A HEPN (higher eukaryote and prokaryote nucleotide binding) nuclease Las1 and a polynucleotide kinase Grc3 assemble into a tetramerase responsible for rRNA maturation. Las1 and Grc3 are highly conserved proteins and have recently been identified as core enzymes involved in processing and removing ITS2 spacer, which is a key step in the synthesis of 60S ribosomal subunit. Recent studies have demonstrated that Las1 is an endoribonuclease that contains a HEPN (higher eukaryote and prokaryote nucleotide binding) domain responsible for rRNA processing. Grc3 is a polynucleotide kinase responsible not only for Las1 nuclease activation, but also for nonspecific phosphorylation of the 5′-OH of the 26S pre-rRNA produced by Las1 cleavage, providing a signal for further processing by Rat1-Rai1 exonuclease.

After screening a large number of crystallization conditions, we successfully obtained well-ordered crystals of the CjLas1 HEPN domain and determined its structure at 1.80 Å resolution using molecular replacement method. The crystallographic asymmetric unit contained three Las1 HEPN molecules (HEPN1, HEPN2, and HEPN3), each of which assumes an all α-helical fold. Analysis of crystal packing and interactions across HEPN-HEPN interfaces suggests that the biological unit of Las1 HEPN domain may contain a homodimer and a monomer. HEPN1 and HEPN2 molecules form a face-to-face dimer related through the preudo-twofold axis, similar to the HEPN dimer in the Las1-Grc3 tetramer structure. Secondly, the catalytic residues in HEPN1 and HEPN2 domains are close to each other to form a compact active center, whereas the catalytic residues in HEPN3 and its symmetry-related molecule remain far apart, presenting two separate catalytic sites. We compared the HEPN domain dimer structures in CjLas1 and CjLas1-Grc3 complex by superposition and observed that significant conformational changes occur in HEPN domains upon Grc3 binding. Remarkably, large conformational changes are observed in the catalytic pocket. In the Grc3-free Las1 structure, the catalytic residues Arg129, His130, and His134 within one HEPN domain are far from the catalytic residues in the other HEPN domain, while in the Grc3-bound structure, the catalytic residues within two HEPN domains are close to each other. These observations indicate that the Grc3 binding not only stabilizes the Las1 HEPN dimer, but also promotes the formation of a more compact catalytic pocket, showing better catalytic activity for specific cleavage of ITS2.

>[3x]MPWKSSDEVVYLKGLFFPADREQISRDELYRQYEEAISLVEMYSSRTRVSHILQSTAHLFSALMMLESFEGGLDDTVRLTASMTIIRFVNGLLDPNQQSQFAIPLHLLAKKIDLPSLFVEFRHSATHDALPSLEMCKTCVDRAIDWVWDHYWDGVLSI>[4x]MSLAEVGSKSVLFVCLGNICRSPIAEAVFRKLVTDEKVSDNWAIDSSAVSDWNVGRPPDPRAVSCLRNHGISTAHKARQITKEDFATFD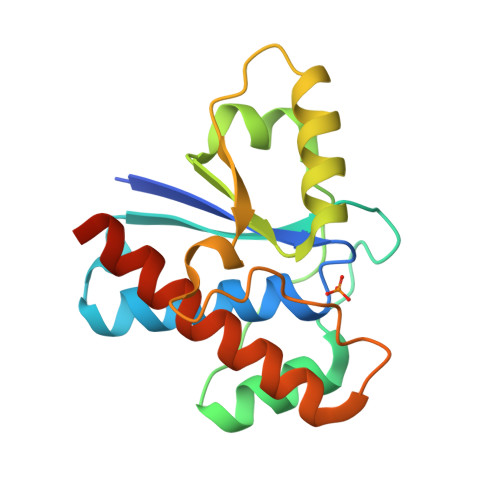YILCMDESNLRDLNRKSNQVKNCKAKIELLGSYDPQKQLIIEDPYYGNDSDFEVVYQQCLRCCKAFLEKTYEGHHHHHH>AGFSMDKANSEAARDGLRAVMEARNVTHLLQQELTEAQKGFQDVEAQAATANHTVMALMASLDAEKAQGQKKVEELEGEITTL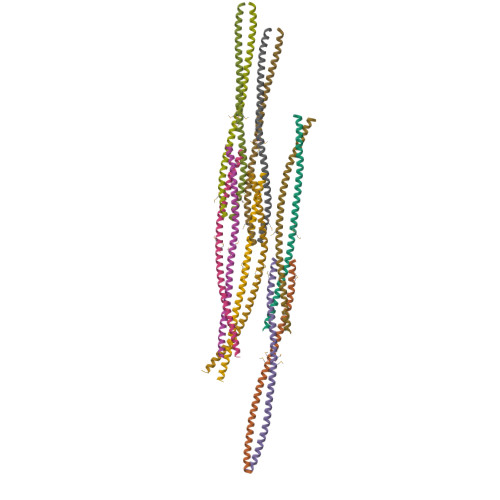NHKLQDASAEVERLRRENQVLSVRIADKKYYPSSQDSS[12x]(2R)-2-(acetylamino)-4-phenylbutanoic acid | C12 H15 N O3 | 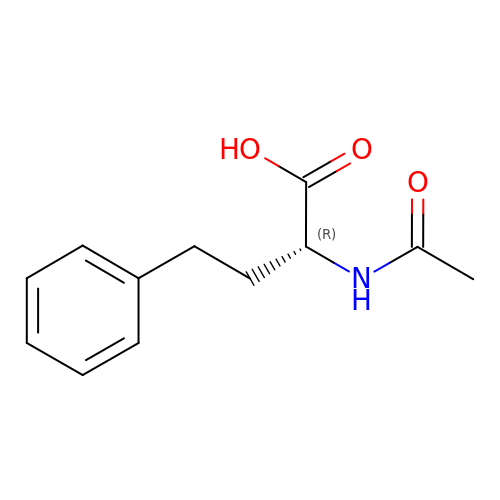CNQZAOFOKXXEOB-LLVKDONJSA-N> MGPVTINNFNYNDPIDNNNIIMMEPPFARGTGRYYKAFKITDRIWIIPERYTFGYKPEDFNKSSGIFNRDVCEYYDPDYLNTNDKKNIFLQTMIKLFNRIKSKPLGEKLLEMIINGIPYLGDRRVPLEEFNTNIASVTVNKLISNPGEVERKKGIFANLIIFGPGPVLNENETIDIGIQNHFASREGFGGIMQMKFCPEYVSVFNNVQENKGASIFNRRGYFSDPALILMHQLIYVLHGLYGIKVDDLPIVPNEKKFFMQSTDAIQAEELYTFGGQDPSIITPSTDKSIYDKVLQNFRGIVDRLNKVLVCISDPNININIYKNKFKDKYKFVEDSEGKYSIDVESFDKLYKSLMFGFTETNIAENYKIKTRASYFSDSLPPVKIKNLLDNEIYTIEEGFNISDKDMEKEYRGQNKAINKQAYEEISKEHLAVYKIQMCKSVKAPGICIDVDNEDLFFIADKNSFSDDLSKNERIEYNTQSNYIENDFPINELILDTDLISKIELPSENTESLTDFNVDVPVYEKQPAIKKIFTDENTIFQYLYSQTFPLDIRDISLTSSFDDALLFSNKVYSFFSMDYIKTANKVVEAGLFAGWVKQIVNDFVIEANKSNTMDKIADISLIVPYIGLALNVGNETAKGNFENAFEIAGASILLEFIPELLIPVVGAFLLESYIDNKNKIIKTIDNALTKRNEKWSDMYGLIVAQWLSTVNTQFYTIKEGMYKALNYQAQALEEIIKYRYNIYSEKEKSNINIDFNDINSKLNEGINQAIDNINNFINGCSVSYLMKKMIPLAVEKLLDFDNTLKKNLLNYIDENKLYLIGSAEYEKSKVNKYLKTIMPFDLSIYTNDTILIEMFNKYNSEILNNIILNLRYKDNNLIDLSGYGAKVEVYDGVELNDKNQFKLTSSANSKIRVTQNQNIIFNSVFLDFSVSFWIRIPKYKNDGIQNYIHNEYTIINCMKNNSGWKISIRGNRIIWTLIDINGKTKSVFFEYNIREDISEYINRWFFVTITNNLNNAKIYINGKLESNTDIKDIREVIANGEIIFKLDGDIDRTQFIWMKYFSIFNTELSQSNIEERYKIQSYSEYLKDFWGNPLMYNKEYYMFNAGNKNSYIKLKKDSPVGEILTRSKYNQNSKYINYRDLYIGEKFIIRRKSNSQSINDDIVRKEDYIYLDFFNLNQEW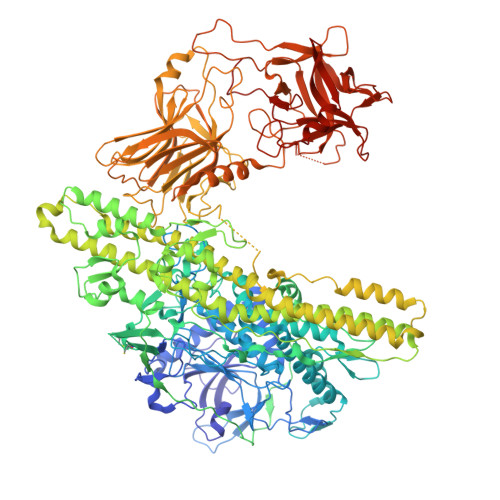RVYTYKYFKKEEEKLFLAPISDSDEFYNTIQIKEYDEQPTYSCQLLFKKDEESTDEIGLIGIHRFYESGIVFEEYKDYFCISKWYLKEVKRKPYNLKLGCNWQFIPKDEGWTEHHHHHHHHHH>MSLAFTKTRSTIGIVAQPVSVEVHLSNGLPSFTMVGLAETAVKESKDRVRSAIINSQFEFPCRKITVNLGPANLPKTGSGFDLPIALGILAASEQIPLTNLANHEFIGELALSGELRGVSAIIPAVLAAHKDNQHLIIANANAAEASLTGHQKVFTANNLREVCDYLCQGTSLQSLPPKPDLLLNNYELDWSDIKGQQHAKNAMVIAACGGHSILLSGAPGSGKTMMAKRFSTLLPELSETQALECAAINSIRGKLPDFREWRLPPFRAPHHTASPVALVGGGNPPKPGEISLAHHGVLFLDELPEFNRQVLETLREPLESGHICISRAAAQIEFPAKFQLIAAMNPCPCGQWGNSQANCMCTPDRISRYLAKLSAPLLDRIDMQVTIHALSQEELIKPNTHLEKQSLAIREKVTKMHEIQMARQDSLNANLNSKTCEMVCELGSEEQLFLREVMSKLKLSARGYHRLLKVSRTIADMNSSKKVLLNHLQQALSYKQNLHLPKHHHHHH[3x]

In Gram-positive Firmicutes, it also has a role in natural transformation, while in Gram-negative bacteria, ComM is the canonical transformation-specific helicase. Comprehensive biochemical characterization of RadA from Escherichia coli, S. pneumoniae, B. subtilis and Thermus thermophilus and ComM from V. cholerae revealed that they are functional homologs during HR. Both RadA and ComM were found to be ring-shaped hexameric DNA motors powered by ATP hydrolysis to direct three-stranded DNA branch migration in vitro. Here, we present and compare the cryoEM (cryogenic electron microscopy) structures of RadA and ComM from S. pneumoniae and Legionella pneumophila, respectively, in interaction with DNA.

Local refinements were also carried out on half of the hexamer and the Lon domain, resulting in an improvement in the quality of the map in these regions. The structure of ComM that is bound to dsDNA was obtained in the presence of the non-hydrolyzable ATP analog AMPPNP, which is located at the interface between two adjacent subunits. Taking the interface between chains C and D as a model, the adenosine nucleotide is coordinated by M226 and K195 of subunit C. The β-phosphate is surrounded by residues 221–225 of subunit C Walker A (residues 218–225). The γ-phosphate is coordinated by the side chains of K224 (lysine piston), T225, and E302 of subunit C. The catalytic glutamate, E302, in subunit C could coordinate a nucleophilic water molecule (not visible in our map) for ATP hydrolysis. In addition, the side chains of R316 (sensor 3 motif) and R463 (arginine finger) of subunit D are also involved in the coordination. In ComM, the H2i loop, which consists of residues 281 to 289, is half the size of its MCM counterpart and prevents the extended hydrophobic interaction along the DNA, instead making a potential contact via a hydrogen bond with Q284. A second region of the protein makes further contact potentially via R366, R369, and K373 residues. Based on the topological arrangement of the ATP-binding site relative to the DNA-binding loops, it is hypothesized that R316, which belongs to the sensor 3 motif, advances the CL1/Ps1β hairpin upon ATP binding.> MATKQAHKRLTKEYKLMVENPPPYILARPNEDNILEWHYIITGPADTPYKGGQYHGTLTFPSDYPYKPPAIRMITPNGRFKPNTRLCLSMSDYHPDTWNPGWSVSTILNGLLSFMTSDEATTGSITTSDHQKKTLARNSISYNTFQNVRFKLIFPEVVQENVETLEKRKLDELPETGG

Ubiquitin-conjugating enzymes (E2) play a crucial role in the attachment of ubiquitin to proteins. A subfamily of E2s, including yeast Ubc6 and human Ube2J2, also mediates noncanonical modification of serines, but the structural determinants for this chemical versatility remain unknown. A rearrangement of the Ubc6/Ube2J2 active site enhances the reactivity of the E2-Ub thioester, facilitating attack by weaker nucleophiles. Moreover, a conserved histidine in Ubc6/Ube2J2 activates a substrate serine by general base catalysis.

To uncover structural determinants of noncanonical E2 activity, we determined two structures of the UBC domain of yeast Ubc6 by X-ray crystallography to resolutions of 1.21 and 1.33 Å, which were virtually identical (RMSD 0.394 Å). First, the loop connecting the four-stranded β-sheet and the active site, which harbors the HPN motif in canonical E2s, is shorter, and contains a conserved GRF motif (called GRF loop). Second, a 12 amino acids long segment, which we will call the Thr-flap, directly connects the crossover helix α2 with helix α4, while the short helix α3 of canonical E2s is lacking. A hydrogen bonding network centered on Arg79 of the GRF motif connects these two segments with each other, the crossover helix α2 and the active site cysteine. In contrast to the published Ube2J2 structure, the active site is well resolved (Figs. 1C and EV1A). It forms a distorted helical structure stabilized by hydrogen bonding between the side chain of Ser91 and Leu88. On top of the active site Cys87 lays an aromatic ring (Tyr93), engaged in a π–cation interaction with Arg85, which itself forms a salt bridge with Asp92. A conserved histidine (His94) points towards the active site Cys87, consistent with a role in the enzymatic mechanism of the ubiquitin transfer reaction.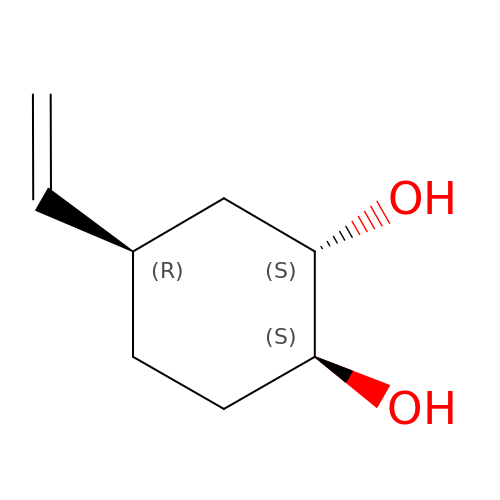(1S,2S,4R)-4-ethenylcyclohexane-1,2-diol | C8 H14 O2 | BSJHRRSHDADBTA-CSMHCCOUSA-N> GPGSMLTYDLIVIGFGKAGKTLAGKLASAGKKVALVERSKAMYGGTCINIGCIPTKTLLVAAEKDLSFEEVIATKNTITGRLNGKNYTTVAGTGVDIFDAEAHFLSNKVIEIQAGDEKQELTAETIVINTGAVSNVLPIPGLATSKNVFDSTGIQSLDKLPEKLGVLGGGNIGLEFAGLYNKLGSKVTVLDTLDTFLPRAEPSIAALAKQYLEEDGIELLQNIHTTEIKNDGDQVLVVTEDETYRFDALLYATGRKPNVEPLQLENTDIELTERGAIKVDKHCQTNVPGVFAVGDVNGGLQFTYISLDDFRVVYSYLAGDGSYTLEDRLNVPNTMFITPALSQVGLTESQAADLKLPYAVKEIPVAAMPRGHVNGDLRGAFKAVVNTETKEILGASIFSEGSQEIINIITVAMDNKIPYTYFTKQIFTHPTLAENLNDLFAI

We recently identified the pneumococcal hypothiocyanous acid reductase (Har), a member of the flavoprotein disulfide reductase enzyme family, and showed that it contributes to the HOSCN tolerance of S. pneumoniae in vitro. Bacterial HOSCN reductases belong to the family of flavoprotein disulfide reductases that, true to their names, utilize a flavin cofactor to transfer electrons from NAD(P)H to a catalytic disulfide within the active site. HOSCN reductases, including Har, MerA, and RclA are expected to form a sulfenylthiocyanate intermediate instead of forming a mixed disulfide. Collectively, our results demonstrate that pneumococcal Har is a highly efficient HOSCN reductase, enabling survival against oxidative host immune defenses.

We determined the X-ray crystal structure of Har in complex with the FAD cofactor to 1.50 Å resolution, highlighting the active site architecture characteristic for this class of enzymes. Har is a monomer in the asymmetric unit of the crystal but is an expected dimer physiologically as for the homologous enzymes MerA and RclA and other characterized flavoprotein disulfide reductases. A minor species (∼2% signal) was present at 4.2 S in the 2 μM sample, which may correspond to a small proportion of monomeric species that exist at lower concentrations. This experiment demonstrates that the single chain in the asymmetric unit of the crystal structure is a result of the crystal symmetry and that Har exists as a homodimer in solution. The monomer of Har comprises four domains that are characteristic of group I flavoprotein disulfide reductases (FAD, NAD(P)H, central and interface). The FAD cofactor is bound as in other flavoprotein disulfide reductases, with the isoalloxazine ring positioned adjacent to the catalytic cysteine residues for electron transfer. Interestingly, our structure reveals two alternative conformations for the conserved residues H425 and E430 of the HXXXXE motif in the active site which have not been previously identified. These residues are in the interface domain and are known to play an important role in the enzyme’s reaction cycle by acting as an acid/base relay, promoting the formation of a reactive thiolate that subsequently reacts with the substrate. The C43 and C48 residues were also solved in two conformations (S-S bound and broken), which could be an artifact whereby exposure to intense X-rays breaks the disulfide bond during data collection. An unexpected area of density was present close to the catalytic C43 residue in the active site of the structure, which has been modelled as a malonate dianion (present in the crystallization condition at 1.2 M). A unique feature of the bacterial HOSCN reductases are two positively charged lysine residues in the active site, which are likely underlying their exceptionally high reactivity towards HOSCN.>TLQPTEAAYIAGFLDGDGSIYAKLEPRPDYKDIKYQVRLAISFIQRKDKFPYLQDIYDQLGKRGNLRKDRGDGIADYTIYGSTHLSIILPDLVPYLRIKKKQANRILHIINLYPQAQKNPSKFLDLVKIVDDVQNLNKRADELKSTNYDRLLEEFLKAGKI[2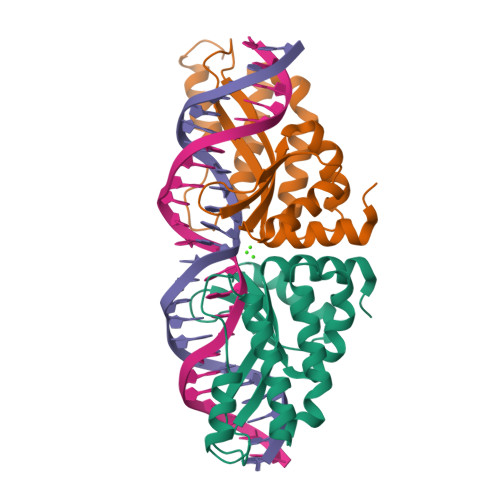x]>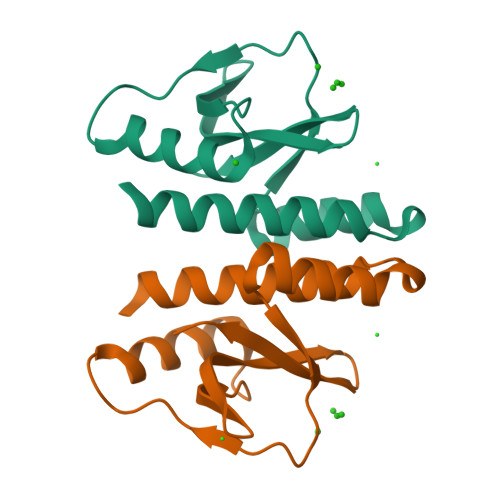 GPGSMFRVIEREPRAQRVALQLVAIVKLTRTALLYSDPDLRRALLQDLESNEGVRVYPREKTDKFKLQPDESVNRLIEHDIRSRLGDDTVIAQSVNDIPGVWISFKIDDDDYWVALDRDQLDTVTG Toxoplasma gondii is one of the most significant parasites that impacts human health, with estimates that as many as one third to one half of the human population are infected. At the Center for Structural Genomics of Infectious Diseases (CSGID), the first Toxoplasma Structural Genomics Pipeline was established. The enzymes selected from the TDR database as small and tractable for expression and crystallization included: phosphoglycerate mutase II (hereafter referred to as PGM), nucleotide diphosphate kinase (NDK), ribulose phosphate 3-epimerase (RPE), ribose-5-phosphate isomerase (RPI), and ornithine aminotransferase (OAT). The genes encoding these enzymes were cloned, proteins expressed and purified, crystallized, and crystal structures were determined.

Ribose-5-phosphate isomerase is the enzyme in the pentose phosphate pathway just upstream of ribulose phosphate 3-epimerase, and it has similar functions, though it catalyzes the transition from ribose-5-phosphate to ribulose-5-phosphate. TgRPI has a larger α/β/α sandwich catalytic domain (residues 1–127 and residues 225–259) with the Rossmann topology and a smaller α/β sandwich oligomerization domain (residues 128–224). Residues 180–186 between strand β8 and a 310-helix (η3), Arg258, and Lys259 are absent in the structure due to their disorder. One D-malate molecule and two chloride ions were modeled to interpret additional electron density. D-malate makes hydrogen bonds with side chains of Lys8, Thr32, and Thr33, and several van der Waals contacts with residues of the phosphate-binding pocket of the active site (Schrödinger SiteMap score 0.97). CL 301/A is bound in the oxyanion hole of the active site and coordinated by main-chain nitrogen atoms of Gly105 and Ala107, side chain carboxyl group of Glu111, and two water molecules, HOH 415 and HOH 433. Applying crystal symmetry operations PISA predicted that TgRPI might exist as unstable dimer (BSA of ~2,430 Å2) or stable dimer (BSA of ~3,340 Å2) in the crystal environment. Homologous RPIs form similar stable dimers and, thus stable TgRPI dimer may be considered biologically relevant. Perhaps the most interesting feature of the determined crystal structure of TgRPI is the disordered region between residues 179–185 that comprises a part of what may appear to be an active site loop. These residues and 310-helix η3 are unique to TgRPI and might be important for catalysis.

> MNPQDKAKQAVGYFAVDTYVRSGMKVGLGTGTTAKFVVERIGQRMQEGSLKDLLCVPTSEATRKQAESLGIPLTTLDGIADCLDVAIDGADEILPPTLGLVKGRGGALLREKMIAAAAKTFIVAADETKLVSNGIGSTGALPVEVVVFSGSHTKRLLSALPSVKRHGGRAEFRKRAGAATGEKNGGQEDIREEDRFVTDNGNYIVDLYFTETVPDLHEMDKELKSIPGVVETGFFLDLASVCLIGKADGSVATLTAERKGENLYFQSAGHHHHHH>[2x]SNAMKTLEKVNYKGFIWPLAVGIVLWLITPWRPGGLSVQAWEMFAIFVATIVGCITKPLPIGGTTLLGMVVTVLVGLAPVKDVVNSKGVVIQTGILSSFGNSAAWLIAMAFIMAHGISKTGLGNRVAYVMIEKFGKRSIGIGYAITGLELMMGALIPSNSARTGGVTWPVVESISKSYDSKPNDPSRKKIGAYLDFMAFHANIL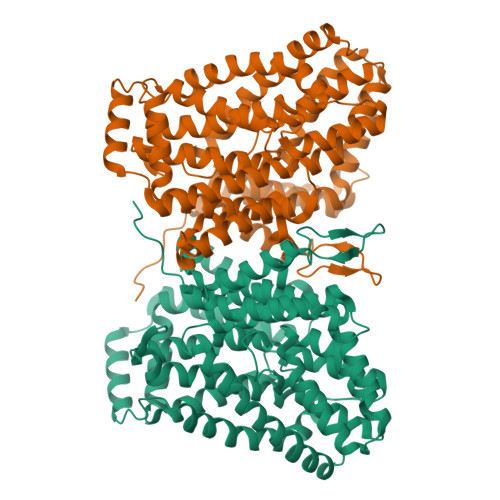STALFITGAAPNLVAQQMAAQKGYQMSWVSWFWAALVPVLVATVIIPLVIYKMYPPEVKETPNAKNWADDKLKEMGPISKPEKIMATVFCLAILLWVLSGFFKIPQLDSAFVAFLAVTLLLITGVLSMEDALHETGAWNILIWLSILIFMAGKLISYGFIAWFAKFIQSEVHGINWGLVLVVLILLMFYTHYFFASGTAHMTALYLPFLTVATAMGAPLGLSAMLLAFTGVINASTTHYANGPASILATTGYVKQSEWWKMNFILGLIYMVIFGIVGTIWMKIIGIW[(2~{R},3~{R},4~{S},5~{S},6~{R})-4-acetamido-6-methyl-3,5-bis(oxidanyl)oxan-2-yl] [[(2~{R},3~{S},5~{R})-5-[5-methyl-2,4-bis(oxidanylidene)pyrimidin-1-yl]-3-oxidanyl-oxolan-2-yl]methoxy-oxidanyl-phosphoryl] hydrogen phosphate  | C18 H29 N3 O15 P2 | 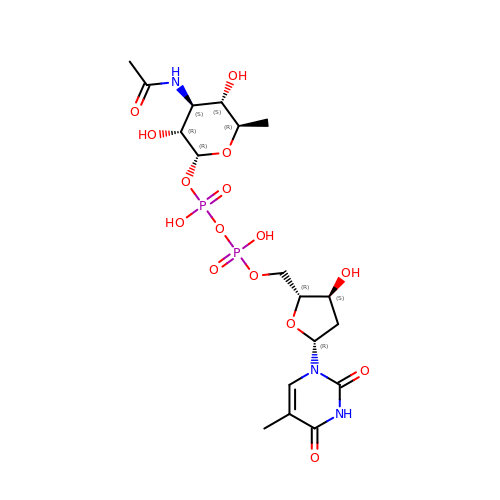CWQDRZJUANNJKC-NMSPNFBVSA-N N-(2-chloropyridin-3-yl)butanamide | C9 H11 Cl N2 O | 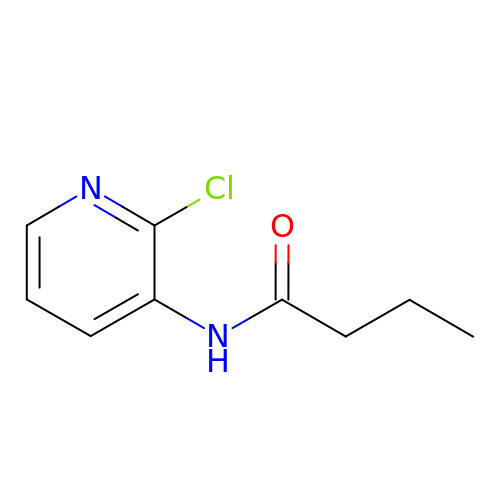UYVCKWSCSBBXER-UHFFFAOYSA-N>AMFNTTPINIDKWLKENEGLLKPPVNNYCLHKGGFTVMIVGGPNERTDYHINPTPEWFYQKKGSMLLKVVDETDAEPKFIDIIINEGDSYLLPGNVPHSPVRFADTVGIVVEQDRPGGENDKIRWYC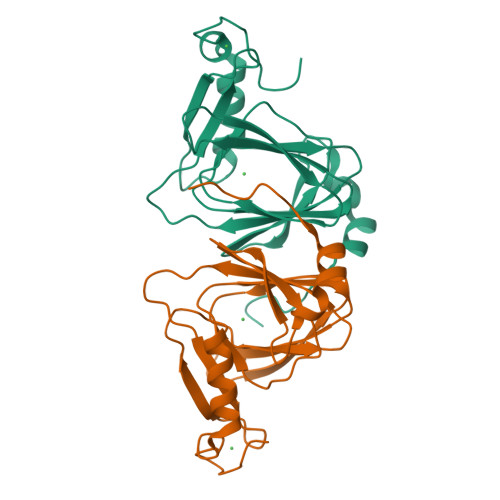SHCRQVVHESELQMLDLGTQVKEAILDFENDVEKRTCFHCKTLNYARPQ[2x]>SMWQINEVVLFDNDPYRILAIEDGQVVWMQISADKGVPQARAELLLMQYLDEGRLVRTDDPYVHLDLEEPSVDSVSFQKREEDYRKILPIINSKDRFDPKVRSELVEHVVQEHKVTKATVYKLLRRYWQRGQTPNALIPDYKNSGAPGERRSATGTAKIGRAREYGKGEGTKVTPEIERLFRLTIEKHLLNQKGTKTTVAYRRFVDLFAQYFPRIPQEDYPTLRQFRYFYDREYPKAQRLKSRVKAGVYKKDVRPLSSTATSQALGPGSRYEIDATIADIYLVDHHDRQKIIGRPTLYIVIDVFSRMITGFYIGFENPSYVVAMQAFVNACSDKTAICAQHDIEISSSDWPCVGLPDVLLADRGELMSHQVEALVSSFNVRVESAPPRRGDAKGIVESTFRTLQAEFKSFAPGIVEGSRIKSHGETDYRLDASLSVFEFTQIILRTILFRNNHLVMDKYDRDADFPTDLPSIPVQLWQWGMQHRTGSLRAVEQEQLRVALLPRRKVSISSFGVNLWGLYYSGSEILREGWLQRSTDIARPQHLEAAYDPVLVDTIYLFPQVGSRVFWRCNLTERSRQFKGLSFWEVWDIQAQEKHNKANAKQDELTKRRELEAFIQQTIQKANKLTPSTTEPKSTRIKQIKTNKKEAVTSERKKRAEHLKPSSS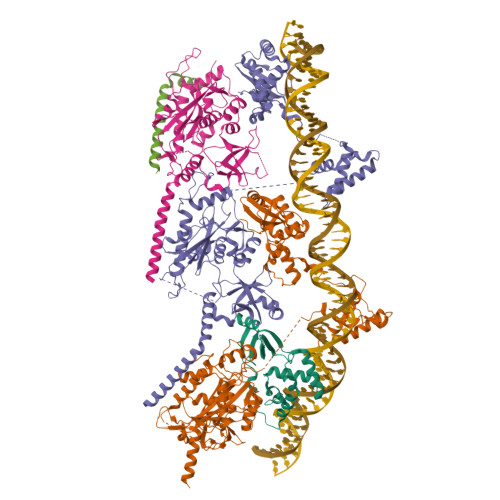GDEAKVIPFNAVEADDQEDYSLPTYVPELFQDPPEKDES[5x]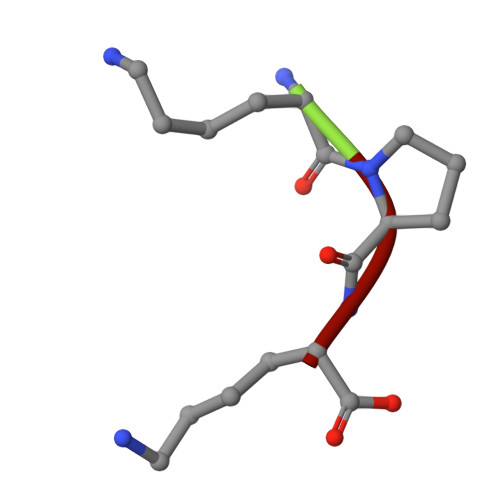> KPK>VPRGSHMKKLLVANRGEIAVRVFRACNELGLSTVAVYAREDEYSVHRFKADESYLIGQGKKPIDAYLDIDDIIRVALESGADAIHPGYGLLSENLEFATKVRAAGLVFVGPELHHLDIFGDKIKAKAAADEAKVPGIPGTNGAVDIDGALEFAKTYGYPVMIKAALGGGGRGMRVARNDAEMHDGYARAKSEAIGAFGSGEIYVEKYIENPKHIEVQILGDRHGNIIHLHERDCSVQRRNQKVIEIAPAVGLSPDFRNEICEAAVKLCKNVGYVNAGTVEFLVKDDKFYFIEVNPRVQVEHTITELITGVDIVQAQILIAQGKDLHREIGLPAQSEIPLLGSAIQCRITTEDPQNGFLPDTGKIDTYRSPGGFGIRLDVGNAYAGYEVTPYFDSLLVKVCTFANEFSDSVRKMDRVLHEFRIRGVKTNIPFLINVIANENFTSGQATTTFIDNTPSLFNFPRLRDRGTKTLHYLSMITVNGFPGIENTEKRHFEEPRQPLLNLEKKKTAKNILDEQGADAVVDYVKNTKEVLLTDTTLRDAHQSLLATRLRLQDMKGIAQAIDQGLPELFSAEMWGGATFDVAYRFLNESPWYRLRKLRKLMPNTMFQMLFRGSNAVGYQNYPDNVIEEFIRVAAHEGIDVFRIFDSLNWLPQM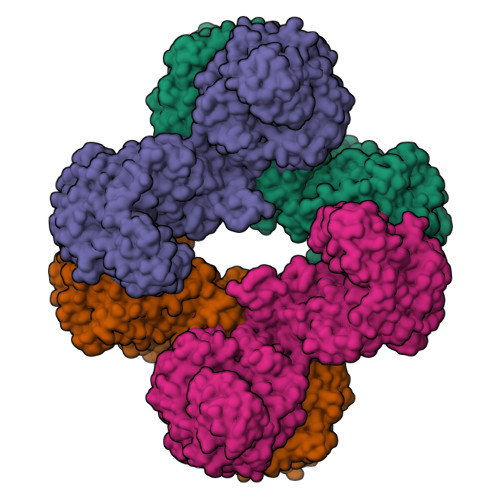EKSIQAVRDNGKIAEATICYTGDILDPSRPKYNIQYYKDLAKELEATGAHILAVKDMAGLLKPQAAYRLISELKDTVDLPIHLHTHDTSGNGIITYSGATQAGVDIIDVATASLAGGTSQPSMQSIYYALEHGPRHASINVKNAEQIDHYWEDVRKYYAPFEAGITSPQTEVYMHEMPGGQYTNLKSQAAAVGLGHRFDEIKQMYRKVNMMFGDIIKVTPSSKVVGDMALFMIQNDLTEEDVYARGNELNFPESVVSFFRGDLGQPVGGFPEKLQKIIVKDKAVITDRPGLHAEKVDFETVKADLEQKIGYEPGDHEVISYIMYPQVFLDYQKMQREFGAVTLLDTPTFLHGMRLNEKIEVQIEKGKTLSIRLDEIGEPDLAGNRVLFFNLNGQRREVVINDQSVQAQVVAKRKAETGNPNQIGATMPGSVLEILVKAGDKVQKGQALMVTEAMKMETTIEAPFDGEIVDLHVVKGEAIQTQDLLIEIN[4x]> GVMTDVHRRFLQLLMTHGVLEEWDVKRLQTHCYKVHDRNATVDKLEDFINNINSVLESLYIEIKRGVTEDDGRPIYALVNLATTSISKMATDFAENELDLFRKALELIIDSETGFASSTNILNLVDQLKGKKMRKKEAEQVLQKFVQNKWLIEKEGEFTLHGRAILEMEQYIRETYPDAVKICNICHSLLI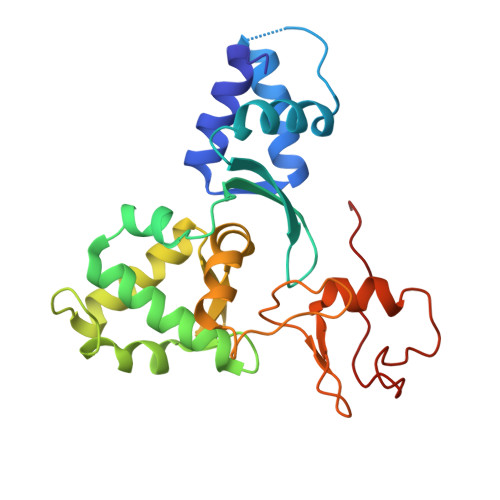QGQSCETCGIRMHLPCVAKYFQSNAEPRCPHCNDYWPHEIPKVFDPE> SNAMTGLFVTLEGPEGAGKSTNRDYLAERLRERGIEVQLTREPGGTPLAERIRELLLAPSDEPMAADTELLLMFAARAQHLAGVIRPALARGAVVLCDR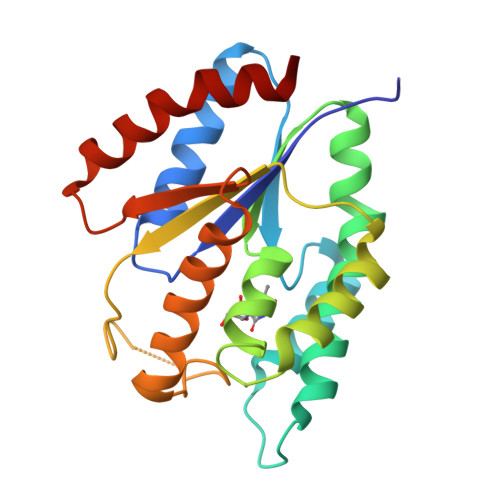FTDATYAYQGGGRGLPEARIAALESFVQGDLRPDLTLVFDLPVEIGLARAAARGRLDRFEQEDRRFFEAVRQTYLQRAAQAPERYQVLDAGLPLAEVQAGLDRLLPNLLERLNG>[4x]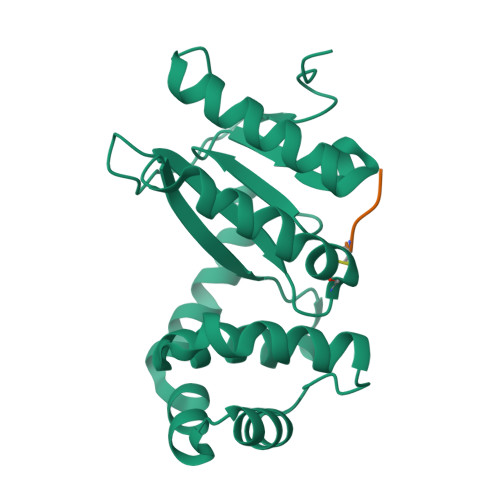SNAAGFAQASPSAPVAGKDFEVMKSPQPVSAPAGKVEVIEFFWYGCPHAYEFEPTIEAWVKKQGDKIAFKRVPVAFRDDFVPHSKLFYALAALGVSEKVTPAVFNAIHKEKNYLLTPQAQADFLATQGVDKKKFLDAYNSFSVQGQVKQSAELLKNYNIDGVPTIVVQGKYKTGPAYTNSLEGTAQVLDFLVKQVQDKKL;>[4x]GFSCGF> MRIGIISVGPGNIMNLYRGVKRASENFEDVSIELVESPRNDLYDLLFIPGVGHFGEGMRRLRENDLIDFVRKHVEDERYVVGVCLGMQLLFEESEEAPGVKGLSLIEGNVVKLRSRRLPHMGWNEVIFKDTFPNGYYYFVHTYRAVCEEEHVLGTTEY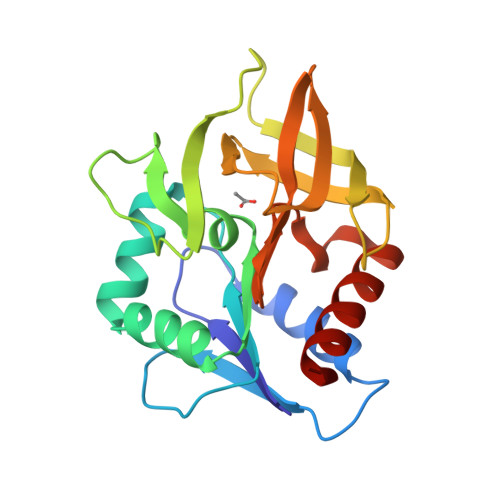DGEIFPSAVRKGRILGFQFHPEKSSKIGRKLLEKVIECSLSRR>[2x]PPRPSSGELWGIHLMPPRILVECLLPNGMIVTLECLREATLITIKHELFKEARKYPLHQLLQDESSYIFVSVTQEAEREEFFDETRRLCDLRLFQPFLKVIEPVGNREEKILNREIGFAIGMPVCEFDMVKDPEVQDFRRNILNVCKEAVDLRDLNSPHSRAMYVYPPNVESSPELPKHIYNKLDKGQIIVVIWVIVSPNNDKQKYTLKINHDCVPEQVIAEAIRKKTRSMLLSSEQLKLCVLEYQGKYILKVCGCDEYFLEKYPLSQYKYIRSCIMLGRMPNLMLMAKESLYSQLPMD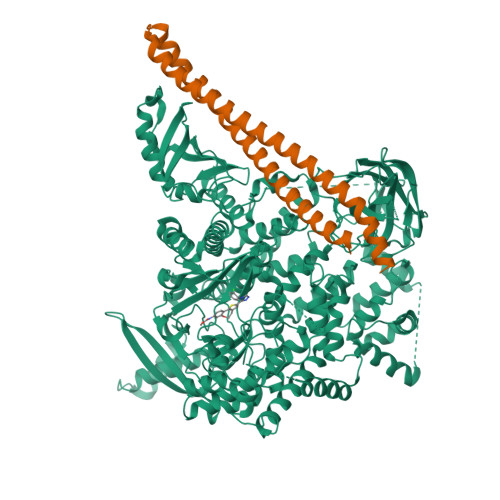CFTMPSYSRRISTATPYMNGETSTKSLWVINSALRIKILCATYVNVNIRDIDKIYVRTGIYHGGEPLCDNVNTQRVPCSNPRWNEWLNYDIYIPDLPRAARLCLSICSVKGRKGAKEEHCPLAWGNINLFDYTDTLVSGKMALNLWPVPHGLEDLLNPIGVTGSNPNKETPCLELEFDWFSSVVKFPDMSVIEEHANWSVSREAGFSYSHAGLSNRLARDNELRENDKEQLKAISTRDPLSEITEQEKDFLWSHRHYCVTIPEILPKLLLSVKWNSRDEVAQMYCLVKDWPPIKPEQAMELLDCNYPDPMVRGFAVRCLEKYLTDDKLSQYLIQLVQVLKYEQYLDNLLVRFLLKKALTNQRIGHFFFWHLKSEMHNKTVSQRFGLLLESYCRACGMYLKHLNRQVEAMEKLINLTDILKQEKKDETQKVQMKFLVEQMRRPDFMDALQGFLSPLNPAHQLGNLRLEECRIMSSAKRPLWLNWENPDIMSELLFQNNEIIFKNGDDLRQDMLTLQIIRIMENIWQNQGLDLRMLPYGCLSIGDCVGLIEVVRNSHTIMQIQCKGGLKGALQFNSHTLHQWLKDKNKGEIYDAAIDLFTRSCAGYCVATFILGIGDRHNSNIMVKDDGQLFHIDFGHFLDHKKKKFGYKRERVPFVLTQDFLIVISKGAQECTKTREFERFQEMCYKAYLAIRQHANLFINLFSMMLGSGMPELQSFDDIAYIRKTLALDKTEQEALEYFMKQMNDAHHGGWTTKMDWIFHTIKQHALN;>YQQDQVVKEDNIEAVGKKLHEYNTQFQEKSREYDRLYEDYTRTSQEIQMKRTAIEAFNETIKIFEEQCQTQERYSKEYIEKFKREGNETEIQRIMHNYEKLKSRISEIVDSRRRLEEDLKKQAAEYREIDKRMNSIKPDLIQLRKTRDQYLMWLTQKGVRQKKLNEWLG[2x]> MKGCSSYLMYSFGGLLSLWILLVSSTNQCTVRYNVADCSHLKLTHIPDDLPSNITVLNLTHNQLRRLPPTNFTRYSQLAILDAGFNSISKLEPELCQILPLLKVLNLQHNELSQISDQTFVFCTNLTELDLMSNSIHKIKSNPFKNQKNLIKLDLSHNGLSSTKLGTGVQLENLQELLLAKNKILALRSEELEFLGNSSLRKLDLSSNPLKEFSPGCFQTIGKLFALLLNNAQLNPHLTEKLCWELSNTSIQNLSLANNQLLATSESTFSGLKWTNLTQLDLSYNNLHDVGNGSFSYLPSLRYLSLEYNNIQRLSPRSFYGLSNLRYLSLKRAFTKQSVSLASHPNIDDFSFQWLKYLEYLNMDDNNIPSTKSNTFTGLVSLKYLSLSKTFTSLQTLTNETFVSLAHSPLLTLNLTKNHISKIANGTFSWLGQLRILDLGLNEIEQKLSGQEWRGLRNIFEIYLSYNKYLQLSTSSFALVPSLQRLMLRRV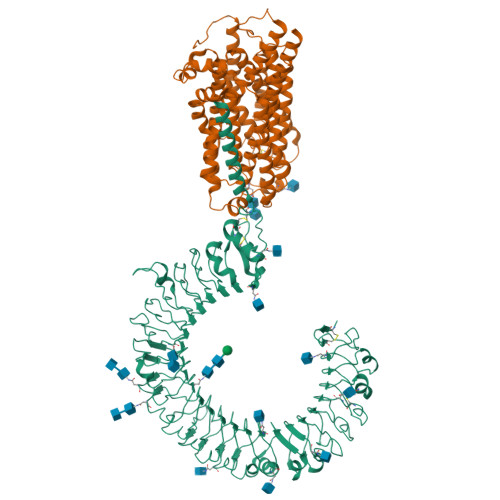ALKNVDISPSPFRPLRNLTILDLSNNNIANINEDLLEGLENLEILDFQHNNLARLWKRANPGGPVNFLKGLSHLHILNLESNGLDEIPVGVFKNLFELKSINLGLNNLNKLEPFIFDDQTSLRSLNLQKNLITSVEKDVFGPPFQNLNSLDMRFNPFDCTCESISWFVNWINQTHTNISELSTHYLCNTPHHYYGFPLKLFDTSSCKDSAPFELLFIISTSMLLVFILVVLLIHIEGWRISFYWNVSVHRILGFKEIDTQAEQFEYTAYIIHAHKDRDWVWEHFSPMEEQDQSLKFCLEERDFEAGVLGLEAIVNSIKRSRKIIFVITHHLLKDPLCRRFKVHHAVQQAIEQNLDSIILIFLQNIPDYKLNHALCLRRGMFKSHCILNWPVQKERINAFHHKLQVALGSRNSAH;> MEVEPPLYPVAGAAGPQGDEDRHGVPDGPEAPLDELVGAYPNYNEEEEERRYYRRKRLGVVKNVLAASTGVTLTYGVYLGLLQMQLILHYDETYREVKYGNMGLPDIDSKMLMGINVTPIAALLYTPVLIRFFGTKWMMFLAVGIYALFVSTNYWERYYTLVPSAVALGMAIVPLWASMGNYITRMSQKYYEYSHYKEQDEQGPQQRPPRGSHAPYLLVFQAIFYSFFHLSFACAQLPMIYFLNNYLYDLNHTLINVQSCGTKSQGILNGFNKTVLRTLPRSKNLIVVESVLMAVAFLAMLMVLGLCGAAYRPTEEIDLRSVGWGNIFQLPFKHVRDFRLRHLVPFFIYSGFEVLFACTGFALGYGVCSMGLERLAYLLIAYSLGASASSVLGLLGLWLPRSVPLVAGAGLHLLLTLSLFFWAPAPRVLQHSWIFYFVAALWGVGSALNKTGLSTLLGILYEDKERQDFIFTIYHWWQAVAIFVVYLGSSLPMKAKLAVLLVTLVAAAASYLWMEQKLQQGLVPRQPRIPKPQHKVRGYRYLEEDNSDESDMEGEQGQGDCAEDEAPQAGPLGAEPAGPCRKPCPYEQALGGDGPEEQ>[2x]GQSVDEMLQKVSAAIEAGQNGQAVSYFRQTIAL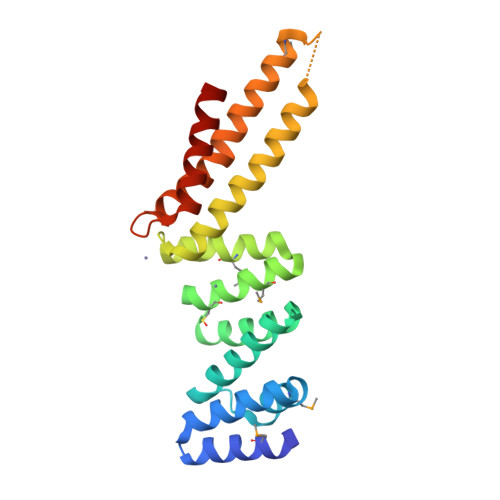NIDRTEMYYWTNVDKNSEISSKLATELALAYKKNRNYDKAYLFYKELLQKAPNNVDCLEACAEMQVCRGQEKDALRMYEKILQLEADNLAANIFLGNYYYLTAEQEKKKLETDYKKLSSPTKMQYARYRDGLSKLFTTRYEKARNSLQKVILRFPSTEAQKTLDKILRIEKEVNR>[12x]MFKIGSVLKQIRQELNYHQIDLYSGIMSKSVYIKVEADSRPISVEELSKFSERLGVNFFEILNRAGMNTKSVNETGKEKLLISKIFTNPDLFDKNFQRIEPKRLTSLQYFSIYLGYI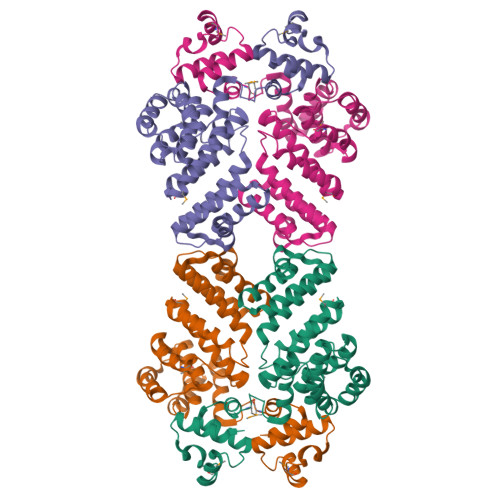SIAHHYNIEVPTFNKTITSDLKHLYDKRTTFFGIDCEIVSNLLNVLPYEEVSSIIKPMYPIVDSFGKDYDLTIQTVLKNALTISIMNRNLKEAQYYINQFEHLKTIKNISINGYYDLEINYLKQIYQFLTDKNIDSYLNAVNIINIFKIIGKEDIHRSLVEELTKISAKEKFTPPKEVTMYYENYVAIENNPIPEIKEQS>MSSLSRELVFLILQFLDEEKFKETVHKLEQESGFFFNMKYFEEKVHAGEWDEVEKYLSGFTKVDDNRYSMKIFFEIRKQKYLEALDRHDRAKAVDILVKDLKVFSTFNEELYKEITQLLTLENFRENEQLSKYGDTKSARSIMLIELKKLIEANP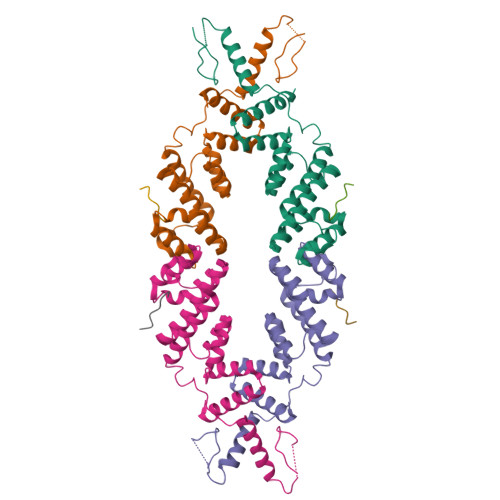LFREKLVFPTLKASRLRTLINQSLNWQHQLCKNPRPNPDIKTLFTDHTCTPPNG[4x];>[4x]DNGLELSLGLS>AATERLSLGSRDVAEALRLSKDIGRLIEAVETAVMPQWQRRELLATVKMLQRRANTAIRKLQMGQAAKKTQELLERHSKGPLIVDTVSAESLSVLVKVVRQLCEQAPSTSVLLLSPQPMGKVLCACQVAQGAMPTFTAEAWALAVCSHMGGKAWGSRVVAQGTGSTTDLEAALSIAQTYALSQLLEHHHHHH[4x]

Consistent with its absence from primate mt tRNAAla sequences, the human mt AlaRS/tRNAAla system was recently shown to be insensitive to a G3:U70 identity element. For the human mt AlaRS/tRNAAla system we show that loss of the G3:U70 identity element was accompanied by a radical reorganization of the recognition mechanism, away from sequence-specific direct readout in the acceptor stem to sequence-unspecific structural readout of the flexible tRNA elbow. The appended C-Ala domain, which plays an auxiliary role in prokaryotic AlaRSs and is dispensable for aminoacylation in the human cytoplasmic AlaRS system, plays a central role as a folding aid for the intrinsically flexible mt tRNA elbow. Fine-tuned induced-fit adaptation selects mt tRNAAla and rejects non-cognate mt tRNAs.

The model suggested two major contact sites between mt C-Ala and mt tRNAAla. The second is formed by helices α2 and α3 of the N-terminal subdomain (aa 783–872). Both helices are lined with highly conserved basic side chains that form an extended patch of positive surface charges. Due to the 3-helix architecture, helices α2 and α3 can move significantly closer to the tRNA than in the prokaryotic complex, allowing direct contacts with the T-stem and V-loop. In particular, the mt AlaRS-specific Gly825 appears to be important for tight association between C-Ala and tRNA and may explain the sensitivity to V-loop size (see above).>APKCIECHINIEMDPVLHDVFKLQVCKQCSKEHPEKYALLTKTECKEDYFLTDPELNDEDLFHRLEKPNPHSGTFARMQLFVRCEVEAFAFKKWGGEE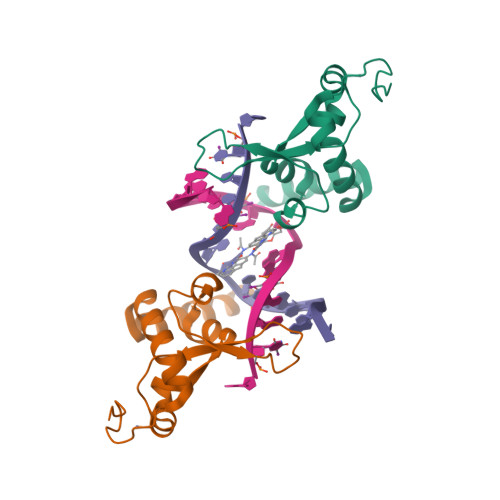GLDEEWQRREEGKAHRR[2x]> PMAAHEASSLYSEEKAKLLREMMAKIEDKNEVLDQFMDSMQLDPETVDNLDAYSHIPPQLMEKCAALSVRPDTVRNLVQSMQVLSGVFTDVEASLKDIRDLLEEDELLEQKFQEAVGQAGAISITSKAELAEVRREWAKYMEVHEKASFTNSELHRAMNLHVGNLRLLSGPLDQVRAALPTPALSPEDKAVLQNLKRILAKVQEMRDQRVSLEQQLRELIQ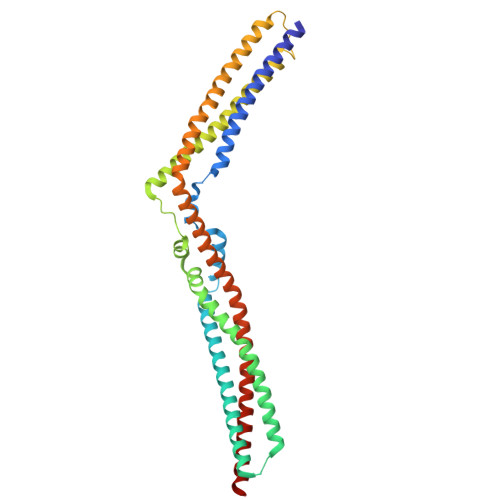KDDITASLVTTDHSEMKKLFEEQLKKYDQLKVYLEQNLAAQDRVLCALTEANVQYAAVRRVLSDLDQKWNSTLQTLVASYEAYEDLMKKSQEGRDFYADLESKVAALLERTQSTCQAREAARQQLLDRELK>[4x]IFNRDPRDH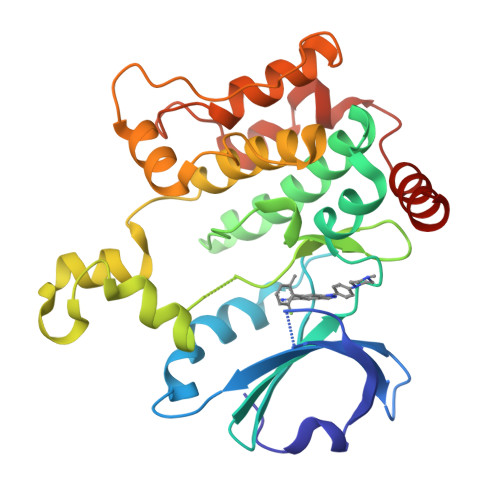YDLLQRLGGGTYGEVFKARDKVSGDLVALKMVKMEPDDDVSTLQKEILILKTCRHANIVAYHGSYLWLQKLWICMEFCGAGSLQDIYQVTGSLSELQISYVCREVLQGLAYLHSQKKIHRDIKGANILINDAGEVRLADFGISAQIGATLARRLAFIGTPYWMAPEVAAVALKGCYNELCDIWSLGITAIELAELQPPLFDVHPLRVLFLMTKSGYQPPRLKEKGKWSAAFHNFIKVTLTKSPKKRPSATKMLSHQLVSQPGLNRGLILDLLDKLKNP>[2x]TTNKPIVLSTFNFGLHANVEAWKVLSKGGKALDAVEKGVRLVEDDPTERSVGYGGRPDR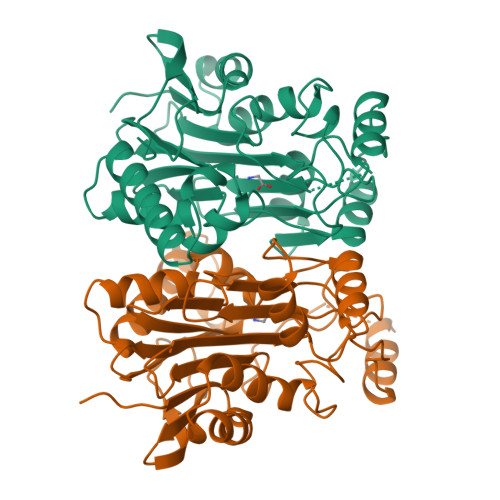DGRVTLDACIMDENYNIGSVACMEHIKNPISVARAVMEKTPHVMLVGDGALEFALSQGFKKENLLTAESEKEWKEWLKTSQYKPIVNIENHDTIGMIALDAQGNLSGACTTSGMAYKMHGRVGDSPIIGAGLFVDNEIGAATATGHGEEVIRTVGTHLVVELMNQGRTPQQACKEAVERIVKIVNRRGKNLKDIQVGFIALNKKGEYGAYCIQDGFNFAVHDQKGNRLETPGFALK>[2x]GSMAPAMEYSTQNGQGEGKKRASVLAIGTTNPEHFILQEDYPDFYFRNTNSEHMTELKEKFKRICVKSHIRKRHFYLTEEILKENQG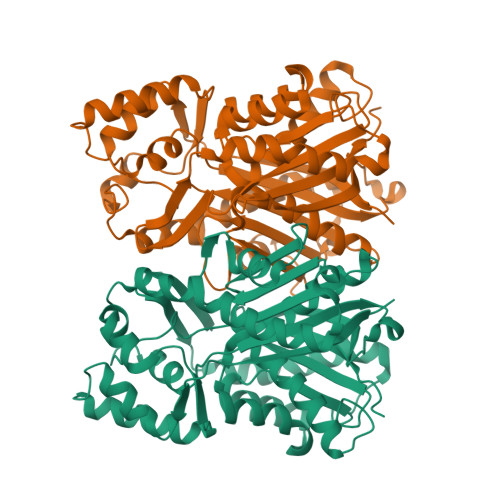IATYGAGSLDARQRILETEVPKLGQEAALKAIAEWGQPISKITHVVFATTSGFMMPGADYVITRLLGLNRTVRRVMLYNQGCFAGGTALRVAKDLAENNEGARVLVVCAENTAMTFHAPNESHLDVIVGQAMFSDGAAALIIGACPDVASGERAVFNILSASQTIVPGSDGAITAHFYEMGMSYFLKEDVIPLFRDNIAAVMEEAFSPLGVSDWNSLFYSIHPGGRGIIDGVAGNLGIKDENLVATRHVLGEYGNMGSACVMFILDELRKSSKVNGKPTTGDGKEFGCLIGLGPGLTVEAVVLQSVPILQ>GSHMASNDLIYQDEHASLQPLEGRTVAVIGYGIQGRAFAANLRDSGVAVRVGNIDDRYFELARAEGHRVTNIAEAVAHADIVLLLIPDEAHGAVFDVDIAPNLRDGALLCVAHGHSLVQGDVRPLPGRDLAMLAPRMYGDPIRRYYLAGQGAPAYFDIVADHTGRARDRVLAIARAVGFTRAGVMALGYRQETFLDLFQEQFLAPALVDLVETGFQVLVERGFNPKAALLEVYGSGEMGKMMLDGADIGLDEVVALQGSPTCQVGYHRWRGRTLPTAVRELAARVLDQIEGGDFSAYLKEQASNDYASLDDARRAALKRPLNVAHAQVRAAFRFPTEAAGGLYQAAQAPADVEPEAAR[2x]

A trait of BP bacteria is a conserved gene cluster coding for the biosynthesis of polyketides (malleicyprols) with a reactive cyclopropanol unit that is critical for virulence. We show that BurG, an unusual NAD+-dependent member of the ketol-acid reductoisomerase family, constructs the strained cyclopropanol ring. A sequence similarity search using BLAST predicted that BurG belongs to the family of ketol-acid reductoisomerases (KARIs; EC 1.1.1.86), well-characterized enzymes that play key roles in the biosynthesis of branched-chain amino acids. Biochemical assays and a suite of eight crystal structures of native and mutated BurG with bound analogues and inhibitors provide snapshots of each step of the complex reaction mechanism, involving a concealed oxidoreduction and a C–S bond cleavage.

We raised crystals of holo-BurG in the absence or presence of 7 as surrogate and solved the structures at a resolution of 1.8 Å and 1.9 Å, respectively. The head region (C1–C3) of all co-crystallized ligands was consistently found to be firmly locked in a conserved binding mode that is facilitated by interactions with the two Mg2+ ions of the enzyme (e for unliganded holo structure).> PAAFSELSLSGLPGHCLTLLAPILRELSEEQDARWLTLIAPPASLTHEWLRRAGLNRERILLLQAKDNAAALALSCEALRLGRSHTVVSWLE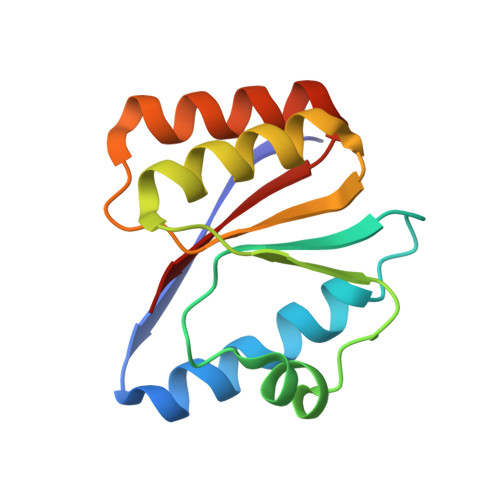PLSRAARKQLSRAAQLGQAQSLNIRLG(3R,5S,9R,23S)-1-[(2R,3S,4R,5R)-5-(6-amino-9H-purin-9-yl)-4-hydroxy-3-(phosphonooxy)tetrahydrofuran-2-yl]-3,5,9-trihydroxy-8,8-dimethyl-10,14-dioxo-23-({[(phenylacetyl)amino]acetyl}amino)-2,4,6-trioxa-18-thia-11,15-diaza-3,5-diphosphatetracosan-24-oic 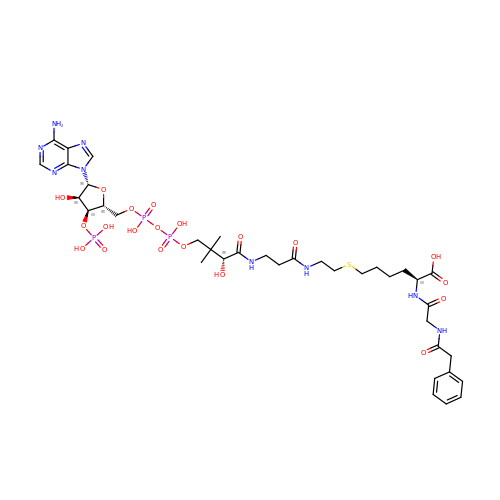acid 3,5-dioxide (non-preferred name) | C37 H56 N9 O20 P3 S | OMXLQYGFXWCBIK-IRRLZKHESA-N>GSHMGGVEVLEVKTGVDSITEVECFLTPEMGDPDEHLRGFSKSISISDTFESDSPNRDMLPCYSVARIPLPNLNEDLTCGNILMWEAVTLKTEVIGVTSLMNVHSNGQATHDNGAGKPVQGTS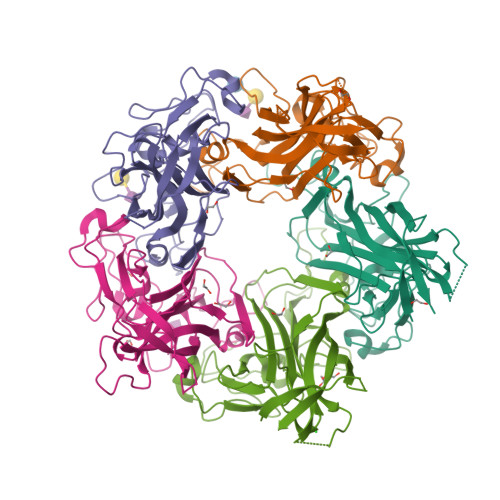FHFFSVGGEALELQGVLFNYRTKYPDGTIFPKNATVQSQVMNTEHKAYLDKNKAYPVECWVPDPTRNENTRYFGTLTGGENVPPVLHITNTATTVLLDEFGVGPLCKGDNLYLSAVDVCGMFTNRSGSQQWRGLSRYFKVQLRKRRVKN[5x]METHYL-[4-(4-PIPERIDINE-1-YLMETHYL-PHENYL)-CYCLOHEXYL]-CARBAMINIC 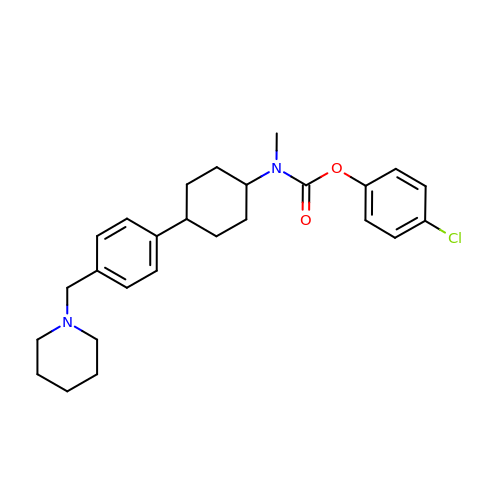ACID-(4-CHLOROPHENYL)-ESTER | C26 H33 Cl N2 O2 | AMKFOVYTEUFMCU-HCGLCNNCSA-N>GANAMGVLISAVGDTDPFRNFHDGALIHIARKYRPEKVILIFSEHTAKKQGNIEKALFSIAPNYEPELIIHDPIISDNEVHIFDVMFQRFSDILQEYYTKEDEFILNLSSATPQIKSALFVINRLNGINVKAVQVSSPEHASNENIGHDNDENIDELIEVNKDNKVNFIDRTIEDNAEKFSQALLKKTARDFIEKFDYKAALDILDQLSDFPNLKSVREEIRDVVNCLSKQDVPKGLRHKKLKEEEQKILSAYLTIELQRERGNVSESFIRIKNLTEFILEDYIKKRYPGLIDEYCEDIQKYYLSLFDYSKLLKATKEFKLKRTIAPIIDMNSSRNKVAHSLSPLDSDAVKQLGIAMKTLKTLVREQYHFSQSDFNFYQDLNKILLTKLN[2x]

Csm6 ribonucleases bind cOA using a CARF (CRISPR-associated Rossmann Fold) domain, resulting in activation of a fused HEPN (Higher Eukaryotes and Prokaryotes Nucleotide binding) ribonuclease domain. Here we characterised the cyclic hexa-adenylate (cA6) activated Csm6’ ribonuclease from the industrially important bacterium Streptococcus thermophilus. StCsm6’ is symmetrical dimer, with each monomer displaying a CARF domain (residues 1–173), a central 6H domain (residues 174–239), and a HEPN domain (residues 240–386). In the dimer, each domain interacts with the equivalent domain in the other monomer, but they cross over each other at the 6H domains to give an ‘X’ arrangement.

We proceeded to solve the structure of StCsm6’ bound to its cA6 activator using X-ray crystallography with data to 1.96 Å resolution. The Fobs-Fcalc map revealed electron density consistent with a molecule of cA6 bound to the StCsm6’ dimer, which was fitted into the model. Upon refinement, it became clear there was actually a mix of species in the binding site, which corresponded to intact cA6 and the two products of cA6 cleavage, linear tri-adenylate molecules containing 2′,3′-cyclic phosphates (A3 > P), with occupancies estimated as 0.50 (cA6) and 0.50 (both A3 > P). Given the symmetrical nature of the StCsm6’ interactions with cA6, cleavage takes place at the identical (but opposite) sides of the cA6 ring to produce two A3 > P molecules. Interestingly, the 2′-OH group of ribose and the phosphate involved in cleavage form minimal interactions with StCsm6’; the 2′-OH forms a hydrogen bond with the backbone amide of N10, and an oxygen atom in the phosphate with T11. Like EiCsm6 (24), the 2′-OH group of ribose and the phosphate involved in cleavage form only two interactions with StCsm6’, and neither of them are sufficiently reactive to play a role in catalysis. This is highly suggestive that StCsm6’ does not assist cleavage by deprotonation of the nucleophile or protonation of the leaving group, and instead it is purely the conformation adopted by cA6 in the binding site that drives catalysis, which would be consistent with a function in slow auto-deactivation of the enzyme. Whilst upon binding of cA6 the CARF and 6H domains appear to tighten with movement towards the dimer interface to enclose cA6, at the opposite side of the protein, in the HEPN domain, a number of the secondary structure elements swing outwards to open up the cavity. This is accompanied by a significant rotation of the CARF domains relative to the HEPN domains, of around 58°, making the overall effect akin to opening a pair of jaws upon binding of cA6 (Video Abstract). The displacement of the secondary structure elements in the HEPN domain causes an increase in distance of ∼6.5 Å at the opening to the active site. In turn, this movement brings the catalytic residues closer together in order to form a functional active site.Nicotinamide adenine dinucleotide (NAD) kinases (NADK) are ubiquitous enzymes, which catalyze the phosphorylation of NAD to nicotinamide adenine dinucleotide phosphate (NADP), which is subsequently reduced to NADPH. Since it is the only known enzyme producing NADP de novo, NAD kinase plays a crucial role in controlling the intracellular balance of NAD(H) and NADP(H) in many cellular metabolic pathways. Therefore, NADK represents a promising target for the development of novel antibiotics with an original mode of action. Here, we describe the synthesis of a series of functionalized diadenosine derivatives based on the chemical structure of NKI1.

The soaking procedure described previously for inhibitor 1 was used to obtain crystals of the target in complex with compounds 2-5. The resulting structures showed the same overall mode of binding to LmNADK1, the ligands occupying both sub-sites A and N of the NAD binding pocket. While compound 3 failed to yield complex with the crystallized target, compound 2 soaking led to a complex with the target. The structure showed a clear change in the orientation of the adenine moiety located in the subsite N (syn vs anti conformation), while that of the adenine moiety in the subsite A was maintained. The purine base flipping positioned the amino end out of the target, while the imidazole ring of the adenine still stacked on Tyr163. However, the N6 spacer arm appears to prevent the usual orientation of the ligand in the subsite N due to van der Waals clashes with neighboring residues, especially Asp150 which is normally hydrogen bonded to the N6 atom. In all three cases, the spacer arms appeared flexible in the crystal structures (weak electron densities) suggesting they are perfectly amenable to column grafting. The introduction of an aminoalkyl chain at position 6 of the adenosine residue located in the N subsite (compounds 2 and 3) led to sharp decrease in inhibitory potency. This finding is consistent with our previous work describing the affinity drop induced by the introduction of a N6-cyclopropylamino group on the adenosine residue located in the subsite N. Introduction of the spacer arm at the 5’-end of the diadenosine derivative (compound 4) resulted in a slightly reduced inhibitory potency as compared to that of inhibitor 1 (NKI1). In contrast, compound 2 showed a different orientation which could explain its increased inhibition constant.

> MKYMITSKGDEKSDLLRLNMIAGFGEYDMEYDDVEPEIVISIGGDGTFLSAFHQYEERLDEIAFIGIHTGHLGFYADWRPAEADKLVKLLAKGEYQKVSYPLLKTTVKYGIGKKEATYLALNESTVKSSGGPFVVDVVINDIHFERFRGDGLCMSTPSGTTAYNKSLGGALMHPSIEAMQLTEMASINNRVYRTIGSPLVFPKHHVVSLQPVNDKDFQISVDHLSILHRDVQEIRYEVSAKKIHFARFRSFPFWRRVHDSFIEDLEHHHHHH> GSHMAGTALKRLMAEYKQLTLNPPEGIV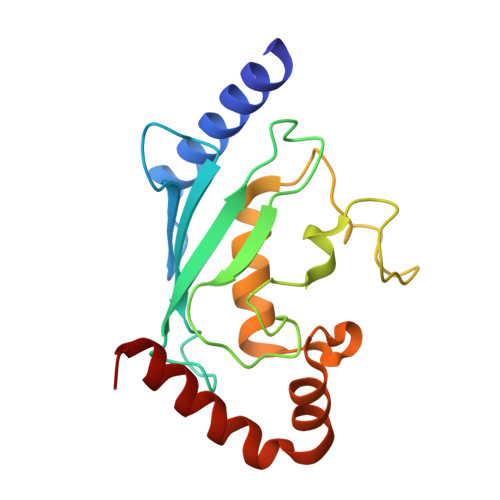AGPMNEENFFEWEALIMGPEDTCFEFGVFPAILSFPLDYPLSPPKMRFTCEMFHPNIYPDGRVCISILHAPGDDPMGYESSAERWSPVQSVEKILLSVVSMLAEPNDESGANVDASKMWRDDREQFYKIAKQIVQKSLGL> MTELNSFQTEEITPFGLKITPQYSDQHIDTLPVEQLKELARKHHLLILRGFKSDLSDHEKYEKYARNWGEIMMWPFGAILDVREHQDATDHVFDNSYMPLHWDGMYKPTIPEFIMFHCAHAPESDQGGRTTFVNTRRVVANATQQQLEQWKNISITYRINKVTHYGGEVHSPLVEEHPDRNGFVIRYNEPAVDGEKFLNKHAIEYHNINPDQVAEFQQDFINILYDKRHLYAHAWKKSDLVIVDNFSLLHGREGFTSKSERHLQRIHIQSNPAFNNQALRS

Two different types of desaturations are employed by iron- and 2-oxoglutarate-dependent (Fe/2OG) enzymes to construct vinyl isonitrile and isocyanoacrylate moieties found in isonitrile-containing natural products. Iron- and 2-oxoglutarate-dependent enzymes catalyze decarboxylation-assisted desaturation and formal dehydrogenation to install vinyl isonitrile (1 and 3) and isocyanoacrylate groups, respectively. Herein, we purify and reconstitute activity of two Fe/2OG enzymes, PvcB and PIsnB, that catalyze 2 and 3 formation in the biosynthesis of paerucumarin and rhabduscin to orchestrate concise chemistries and to establish governing factors utilized for vinyl isonitrile and isocyanoacrylate moieties installation. While the active site and substrate binding of PIsnB and PvcB are highly similar, different reaction products (2 and 3) are generated by PvcB and PIsnB, respectively.

The ternary complex (PlsnB•Mn•4) was prepared for structure determination by co-crystallization approach. The diffraction data were collected to a resolution of 1.98 Å, with each asymmetric unit containing one molecule of PIsnB in the space group P212121. The final model shows that PIsnB exists as a monomer which is consistent with the oligomeric state determined by gel filtration. Analogous to other Fe/2OG enzymes, PlsnB has two four-stranded β-sheet in the center, a.k.a., jelly roll or Swiss roll fold. The metal ion is coordinated by His101, Asp103, His250, and three water molecules. The benzene ring of 4 locates in a hydrophobic pocket formed by Tyr106, Ile159, Trp102, and Met105. While the ample space of the hydrophobic pocket allows the rotation of the benzene ring, the π-π stacking of the phenyl ring of 4 and His101 may result in a preferred orientation as the observed in the crystal structure. Namely, the carboxylate is anchored by Arg265, which has a cation-π interaction with Trp74 with a distance of 3.5 Å to the indole ring. Since the carboxylate group has hydrogen bonds with Gly104 and an iron-coordinated water, such orientation enforces the isonitrile moiety to point away from the iron center. No apparent interaction can be identified within 5 Å of the isonitrile group.>MRYRKGARDTAFLVLYRWDLRGENPGELFKEVVEEKNIKNKDAYEYAKKLVDTAVRHIEEIDSIIEKHLKGWSIDRLGYVERNALRLGVAELIFLKSKEPGRVFIDIVDLVKKYADEKAGK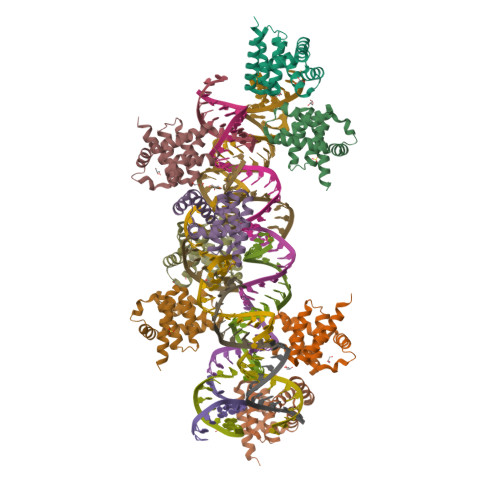FVNGVLSAIYKAYITSSKEEKPSLKSE[8x]>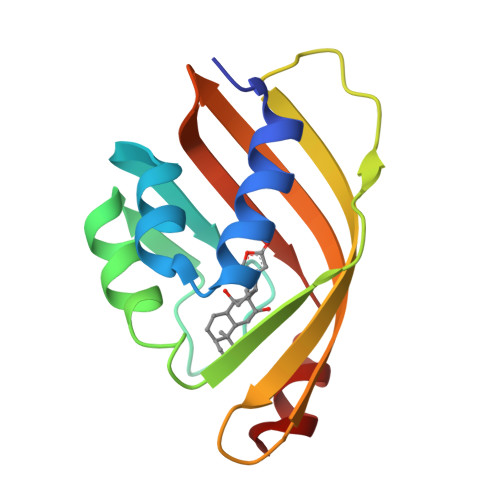GSSMNAKEILVHSLRLLENGDARGWCDLFHPEGVLEYPYAPPGWKTRFEGRETIWAHMRLHPEHVTWRFTDVQFYETADPDLAIGEYHGDGVVTVSGGKYAADYITVLRTRDGQILLLRVFWNPLRILEAAG[4x]>[2x]FVNKDQIAKDVKQFYDQALQQAVVDDDANNAKAVVKTFHETLDCCGSS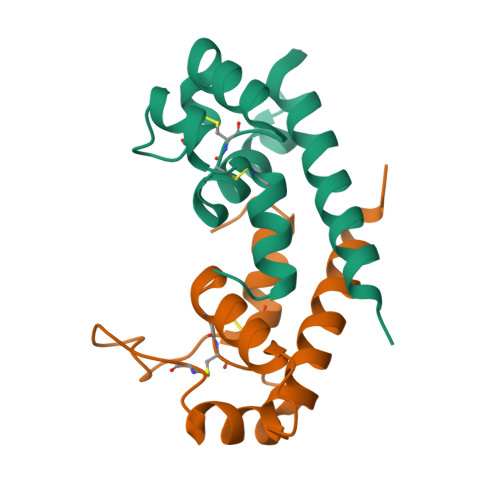TLTALTTSVLKNNLCPSGSNIISNLFKEDCHQKIDDLFSGKH Specialized protein transport systems—known as type VII secretion systems (T7SSs)—are central to the virulence of this pathogen, and are also crucial for nutrient and metabolite transport across the mycobacterial cell envelope. Mycobacterium tuberculosis encodes five homologous, but functionally distinct, T7SSs that are designated ESX-1 to ESX-5. These systems translocate a number of effector proteins across the unique and impermeable diderm cell envelope. Here we reconstituted the ESX-5 T7SS of M. tuberculosis H37Rv in M. smegmatis to obtain a structural view of the entire T7SS membrane complex from this human pathogen.

Cryo-electron microscopy (cryo-EM) analysis of the M. tuberculosis ESX-5 complex purified in the presence of ADP–AlF3 showed clear hexameric particles. We performed an ab initio reconstruction without symmetry enforcement that yielded an average resolution of approximately 4 Å, which improved to an overall resolution of approximately 3.5 Å after further data processing; this allowed us to build around 78% of the stable complex de novo. The intact machinery comprises EccB5, EccC5, EccD5, EccE5 and MycP5 with a 6:6:12:6:3 stoichiometry resulting in a 2.32-MDa complex that is anchored in the inner membrane through 165 transmembrane helices (TMHs). The membrane assembly is best described as a trimer of dimers, in which each dimer comprises a single copy of MycP5 and two protomers each of one copy of EccB5, EccC5, EccE5 and two copies of EccD5. In the intact ESX-5 complex, the angle between protomers at the membrane level differs by about 0.5°, from 59.7° between protomers of one dimer to 60.2° between protomers of adjacent dimers. However, at the cytosolic level these angles differ by more than 10° (from 65.3° to 54.7°). Beneath the EccB5–MycP5 chamber, dimers of the EccC5 ATPase assemble into three bundles of four transmembrane helices each, which together seal the potential central secretion channel. At the very centre of the complex, one TMH of each bundle contributes to the formation of a pyramidal assembly that aligns with the periplasmic chamber. Individual cytoplasmic EccC5 domains adopt two distinctive conformations that probably reflect different secretion states. Our work provides a fully assembled structure of the ESX-5 inner-membrane complex of M. tuberculosis.

>[6x]MAEESRGQRGSGYGLGLSTRTQVTGYQFLARRTAMALTRWRVRMEIEPGRRQTLAVVASVSAALVICLGALLWSFISPSGQLNESPIIADRDSGALYVRVGDRLYPALNLASARLITGRPDNPHLVRSSQIATMPRGPLVGIPGAPSSFSPKSPPASSWLVCDTVATSSSIGSLQGVTVTVIDGTPDLTGHRQILSGSDAVVLRYGGDAWVIREGRRSRIEPTNRAVLLPLGLTPEQVSQARPMSRALFDALPVGPELLVPEVPNAGGPATFPGAPGPIGTVIVTPQISGPQQYSLVLGDGVQTLPPLVAQILQNAGSAGNTKPLTVEPSTLAKMPVVNRLDLSAYPDNPLEVVDIREHPSTCWWWERTAGENRARVRVVSGPTIPVAATEMNKVVSLVKADTSGRQADQVYFGPDHANFVAVTGNNPGAQTSESLWWVTDAGARFGVEDSKEARDALGLTLTPSLAPWVALRLLPQGPTLSRADALVEHDTLPMDMTPAELVVPK;>MKRGFARPTPEKPPVIKPENIVLSTPLSIPPPEGKPWWLIVVGVVVVGLLGGMVAMVFASGSHVFGGIGSIFPLFMMVGIMMMMFRGMGGGQQQMSRPKLDAMRAQFMLMLDMLRETAQESADSMDANYRWFHPAPNTLAAAVGSPRMWERKPDGKDLNFGVVRVGVGMTRPEVTWGEPQNMPTDIELEPVTGKALQEFGRYQSVVYNLPKMVSLLVEPWYALVGEREQVLGLMRAIICQLAFSHGPDHVQMIVVSSDLDQWDWVKWLPHFGDSRRHDAAGNARMVYTSVREFAAEQAELFAGRGSFTPRHASSSAQTPTPHTVIIADVDDPQWEYVISAEGVDGVTFFDLTGSSMWTDIPERKLQFDKTGVIEALPRDRDTWMVIDDKAWFFALTDQVSIAEAEEFAQKLAQWRLAEAYEEIGQRVAHIGARDILSYYGIDDPGNIDFDSLWASRTDTMGRSRLRAPFGNRSDNGELLFLDMKSLDEGGDGPHGVMSGTTGSGKSTLVRTVIESLMLSHPPEELQFVLADLKGGSAVKPFAGVPHVSRIITDLEEDQALMERFLDALWGEIARRKAICDSAGVDDAKEYNSVRARMRARGQDMAPLPMLVVVIDEFYEWFRIMPTAVDVLDSIGRQGRAYWIHLMMASQTIESRAEKLMENMGYRLVLKARTAGAAQAAGVPNAVNLPAQAGLGYFRKSLEDIIRFQAEFLWRDYFQPGVSIDGEEAPALVHSIDYIRPQLFTNSFTPLEVSVGGPDIEPVVAQPNGEVLESDDIEGGEDEDEEGVRTPKVGTVIIDQLRKIKFEPYRLWQPPLTQPVAIDDLVNRFLGRPWHKEYGSACNLVFPIGIIDRPYKHDQPPWTVDTSGPGANVLILGAGGSGKTTALQTLICSAALTHTPQQVQFYCLAYSSTALTTVSRIPHVGEVAGPTDPYGVRRTVAELLALVRERKRSFLECGIASMEMFRRRKFGGEAGPVPDDGFGDVYLVIDNYRALAEENEVLIEQVNVIINQGPSFGVHVVVTADRESELRPPVRSGFGSRIELRLAAVEDAKLVRSRFAKDVPVKPGRGMVAVNYVRLDSDPQAGLHTLVARPALGSTPDNVFECDSVVAAVSRLTSAQAPPVRRLPARFGVEQVRELASRDTRQGVGAGGIAWAISELDLAPVYLNFAENSHLMVTGRRECGRTTTLATIMSEIGRLYAPGASSAPPPAPGRPSAQVWLVDPRRQLLTALGSDYVERFAYNLDGVVAMMGELAAALAGREPPPGLSAEELLSRSWWSGPEIFLIVDDIQQLPPGFDSPLHKAVPFVNRAADVGLHVIVTRTFGGWSSAGSDPMLRALHQANAPLLVMDADPDEGFIRGKMKGGPLPRGRGLLMAEDTGVFVQVAATEVRR[6x];>[12x]MTAVADAPQADIEGVASPQAVVVGVMAGEGVQIGVLLDANAPVSVMTDPLLKVVNSRLRELGEAPLEATGRGRWALCLVDGAPLRATQSLTEQDVYDGDRLWIRFIADTERRSQVIEHISTAVASDLSKRFARIDPIVAVQVGASMVATGVVLATGVLGWWRWHHNTWLTTIYTAVIGVLVLAVAMLLLMRAKTDADRRVADIMLMSAIMPVTVAAAAAPPGPVGSPQAVLGFGVLTVAAALALRFTGRRLGIYTTIVIIGALTMLAALARMVAATSAVTLLSSLLLICVVAYHAAPALSRRLAGIRLPVFPSATSRWVFEARPDLPTTVVVSGGSAPVLEGPSSVRDVLLQAERARSFLSGLLTGLGVMVVVCMTSLCDPHTGQRWLPLILAGFTSGFLLLRGRSYVDRWQSITLAGTAVIIAAAVCVRYALELSSPLAVSIVAAILVLLPAAGMAAAAHVPHTIYSPLFRKFVEWIEYLCLMPIFPLALWLMNVYAAIRYR;>[3x]MQRFGTGSSRSWCGRAGTATIAAVLLASGALTGLPPAYAISPPTIDPGALPPDGPPGPLAPMKQNAYCTEVGVLPGTDFQLQPKYMEMLNLNEAWQFGRGDGVKVAVIDTGVTPHPRLPRLIPGGDYVMAGGDGLSDCDAHGTLVASMIAAVPANGAVPLPSVPRRPVTIPTTETPPPPQTVTLSPVPPQTVTVIPAPPPEEGVPPGAPVPGPEPPPAPGPQPPAVDRGGGTVTVPSYSGGRKIAPIDNPRNPHPSAPSPALGPPPDAFSGIAPGVEIISIRQSSQAFGLKDPYTGDEDPQTAQKIDNVETMARAIVHAANMGASVINISDVMCMSARNVIDQRALGAAVHYAAVDKDAVIVAAAGDGSKKDCKQNPIFDPLQPDDPRAWNAVTTVVTPSWFHDYVLTVGAVDANGQPLSKMSIAGPWVSISAPGTDVVGLSPRDDGLINAIDGPDNSLLVPAGTSFSAAIVSGVAALVRAKFPELSAYQIINRLIHTARPPARGVDNQVGYGVVDPVAALTWDVPKGPAEPPKQLSAPLVVPQPPAPRDMVPIWVAAGGLAGALLIGGAVFGTATLMRRSRKQQ> GPLGSMDSSQLHVAIVSSPGMGHLIPVLVLGNRLATHHNIKITILAITTTSSSAETEFLKKTTLTNEEKTIEIIPVPSVDISHLINSSTKIFTQLRLLVREALPKIHSTIASMTHRPDALIVDIFCTQILPIAEEFNISKYTYHPTTAWTLALAIYCQVFDKEIEGEYVELKEPLKIPGCKALRPDDVVDPLLDRSDQQYEEYVKLGKEYTDFDGILINTWEDLEPETINALRYNEKLRLLLKVPVFPIGPLRRKVETTLNDEVIQWLDKQNNESVLFVSFGSGGTLSTKQMTELAWG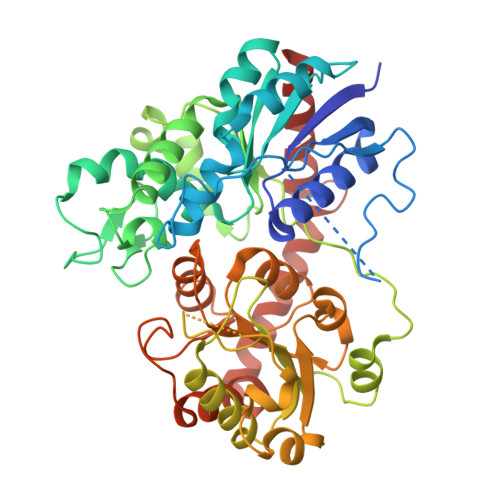LELSQQKFVWVVRPPSDGDADSAYLNSAGKDTRDMSEYLPEGFLTRTKDMGLVVPMWANQVEILSHSSVGGFLTHCGWNSTVESLTNGVPMIAWPLHAEQKMNAAMLTEELGVAIRPAVLPTKKLVKREEIQGMVRILMQTKEGKRIKEKAKKLKKSAENALSDGGSSYNSICELVKDIRSR>[2x]MGSGSSSYRPKAIYLDIDGRIQKVIFSKYCNSSDIMDLFCIATGLPRNTTISLLTTDD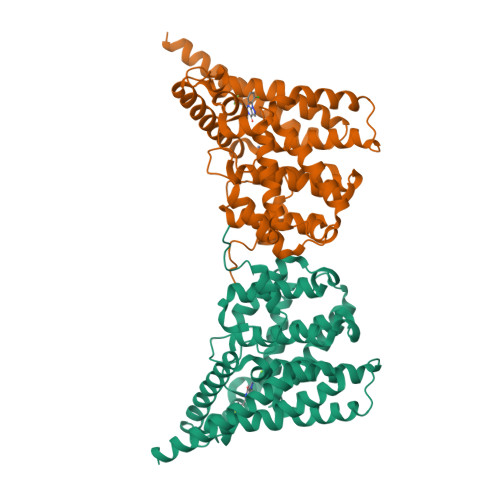AMVSIDPTMPANSERTPYKVRPVAIKQLSEREELIQSVLAQVAEQFSRAFKINELKAEVANHLAVLEKRVELEGLKVVEIEKCKSDIKKMREELAARSSRTNCPCKYSFLDNHKKLTPRRDVPTYPKYLLSPETIEALRKPTFDVWLWEPNEMLSCLEHMYHDLGLVRDFSINPVTLRRWLFCVHDNYRNNPFHNFRHCFCVAQMMYSMVWLCSLQEKFSQTDILILMTAAICHDLDHPGYNNTYQINARTELAVRYNDISPLENHHCAVAFQILAEPECNIFSNIPPDGFKQIRQGMITLILATDMARHAEIMDSFKEKMENFDYSNEEHMTLLKMILIKCCDISNEVRPMEVAEPWVDCLLEEYFMQSDREKSEGLPVAPFMDRDKVTKATAEIGFIKFVLIPMFETVTKLFPMVEEIMLQPLWESRDRYEELKRIDDAMKELQKKTDSLTSGATEKSRERSRDVKNSEGDCA> QGGGEDSLGMEVGYRLIPMVDFQQDGELLGRIRSIRKKFAQDMGFLPPVVHIRDNMDLQPARYRILMKGVEIGSGDAYPGRWLAINPGTAAGTLPGEKTVDPAFGLDAIWIESALKEQAQIQGFTVVEASTVVATHLNHLIGQFSAELFGRQEAQQLLDRVSQ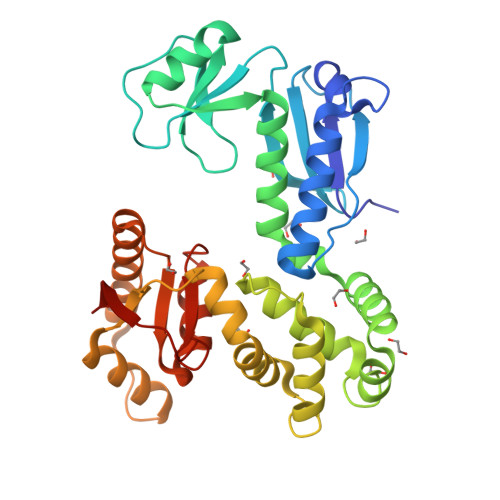EMPKLTEDLVPGVVTLTTLHKVLQNLLAEKVPIRDMRTILETLAEHAPLQSDPHELTAVVRVALGRAITQQWFPGNEEVQVIGLDTALERLLLQALQGGGGLEPGLADRLLAQTQEALSRQEMLGAPPVLLVNHALRPLLSRFLRRSLPQLVVLSNLELSDNRHIRMTATIGGK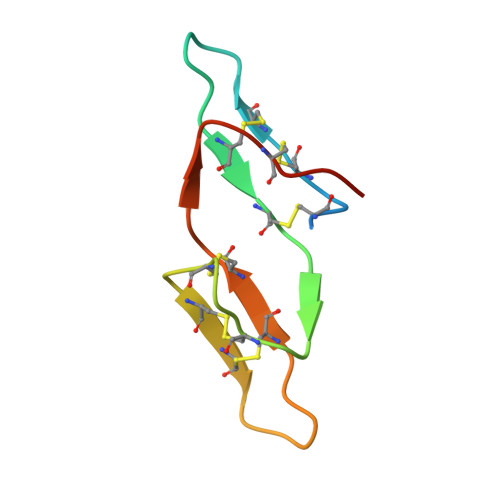> TKSTTTACCDFCPCTRSIPPQCQCTDVREKCHSACKSCLCTRSFPPQCRCYDITDFCYPSCS(1S,2S,3S,6R)-4-(hydroxymethyl)-6-(octylamino)cyclohex-4-ene-1,2,3-triol | C15 H29 N O4 | 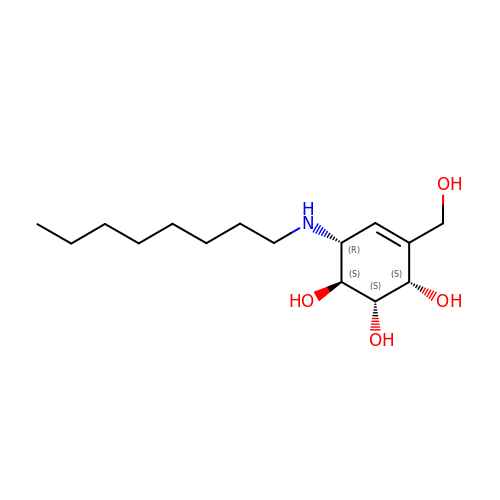UPZUHYMBTUUPML-QPSCCSFWSA-N>[2x]GPMGEDDLIFRVGTKGRNKGEFTNLQGVAASTNGKILIADSNN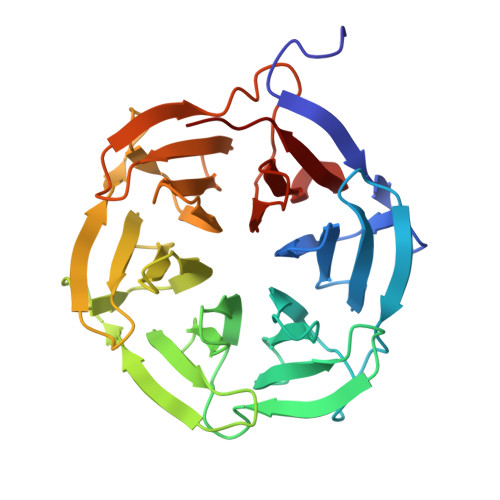QCVQIFSNDGQFKSRFGIRGRSPGQLQRPTGVAVHPSGDIIIADYDNKWVSIFSSDGKFKTKIGSGKLMGPKGVSVDRNGHIIVVDNKACCVFIFQPNGKIVTRFGSRGNGDRQFAGPHFAAVNSNNEIIITDFHNHSVKVFNQEGEFMLKFGSNGEGNGQFNAPTGVAVDSNGNIIVADWGNSRIQVFDGSGSFLSYINTSADPLYGPQGLALTSDGHVVVADSGNHCFKVYRYLQ>[4x]MARLDKSKVINSALELLNEVGIEGLTTRKLAQKLGVEQPT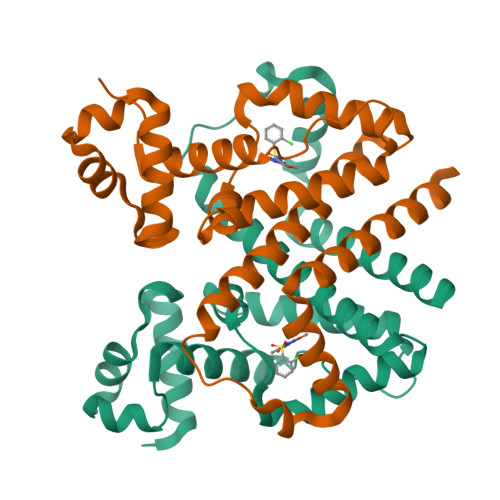LYWHVKNKRALLDALAIEMHDRHQTHYLPLEGESWQDFLRNFAKSMRLALLSHRDGAKVSLGTRWTEQQYETAENMLAFLTQQGFSLENALYATDAVRVFTLGAVLLDQEQQVAKEERETPTPDSMPPLLRQAWELKVHQGAEPAFLFGLELIIAGLEKQLKRESGS>MTDAVSDALHTRHDSAPSAVKGTIIVSGGSQGLGLTTVRCFLEAGYNVATFSRRESPAVTELSERADFHWQALDCTDYSALTAFVQQVEKRFGGLDGLVNNAATGVEGILSTMRVADIDSALDINLKGQLYLTKLVTAKLLKRGAGSVVNVSSINALRGHSGLTVYSATKAAMDGLTRSLAKELGPRGIRVNSVSPGYFSSDMVKDLSPQTLSRIERRTPLGRLGTQQEVADLILYLVDRGTFVTGQNIA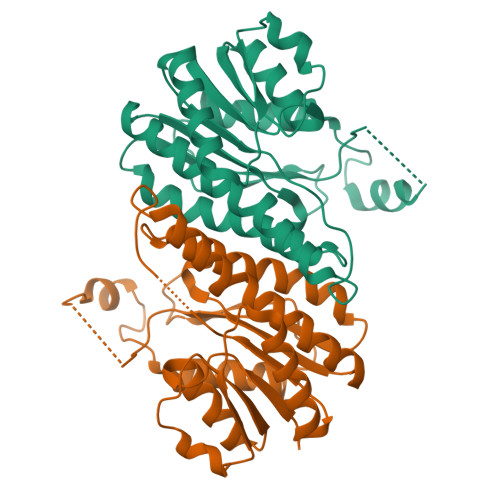VDGGFTC[2x]> EGGDFVVGMVTDSGDIDDKSFNQQVWEGISRFAQENNAKCKYVTASTDAEYVPSLSAFADENMGLVVACGSFLVEAVIETSARFPKQKFLVIDAVVQD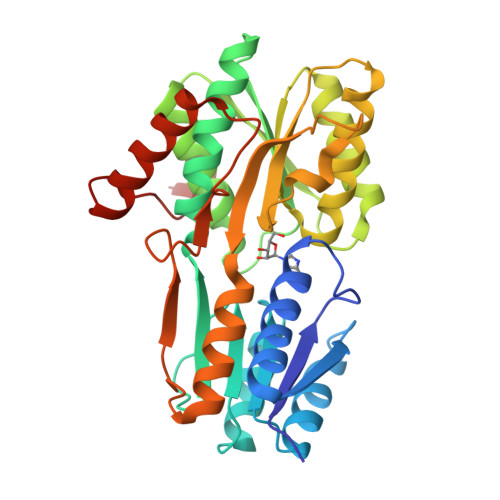RDNVVSAVFGQNEGSFLVGVAAALKAKEAGKSAVGFIVGMELGMMPLFEAGFEAGVKAVDPDIQVVVEVANTFSDPQKGQALAAKLYDSGVNVIFQVAGGTGNGVIKEARDRRLNGQDVWVIGVDRDQYMDGVYDGSKSVVLTSMVKRADVAAERISKMAYDGSFPGGQSIMFGLEDKAVGIPEENPNLSSAVMEKIRSFEEKIVSKEIVVPVRSARMMN>MAIELNVGRKVTVTVPGSSANLGPGFDTLGLALSVYDTVEVEIIPSGLEVEVFGEGQGEVPLDGSHLVVKAIRAGLKAADAEVPGLRVVCHNNIPQSRGLGSSAAAAVAGVAAANGLADFPLTQEQIVQLSSAFEGHPDNAAASVLGGAVVSWTNLSIDGKSQPQYAAVPLEVQDNIRATALVPNFHASTEAVRRVLPTEVTHIDARFNVSRVAVMIVALQQRPDLLWEGTRDRLHQPYR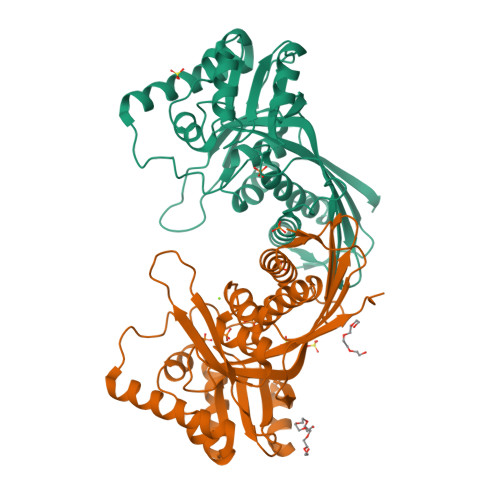AEVLPITSEWVNRLRNRGYAAYLSGAGPTAMVLSTEPIPDKVLEDARESGIKVLELEVAGPVKVEVNQPHHHHHH[2x]pyridine-3-sulfonic 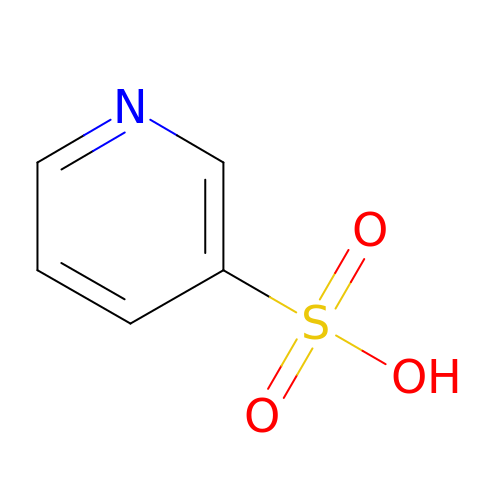acid | C5 H5 N O3 S | DVECLMOWYVDJRM-UHFFFAOYSA-N> MADLSLARQRLTDESVNEAPRAYDANMELVIVAEYPEGQCKSFHFANPFVIKGVIKSSELMWDIDNGHQMSEYELQRSINGYAASHSNMRQRSAINRIPKKLSFYLRGNVDWNKASIDIRG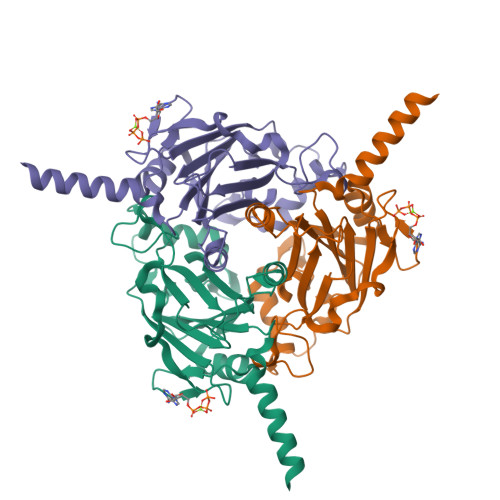PTGLSMRQTEEYSLDRIRPPCSYKRNKFVDLPSCGGRCEKAWYVELDGRPVSIAVIVPRNMHNGINLYAGPLLGNVIEGLDTVPECTQWFDNAPELYAYHASNYGMTMLDQFSVIH> MAPTPKYTFTERAAAGNLSDAEILNSNNPTGSELPDESDVVVGGAGIHGLIYALHASKYKPNNLKISVIEKNTRPGYKIGESTLPIFYTWCKLHGISAAYLLRLFGLKDGLCFYFLDRENQGQYTDFCSVGAPGLVLASLQIERPMSELLFTILAQRNGVNVYHGREVDFKSTVVQGGGQGNKIAVSRGKYDSTPKTIDSALFVDATGRFRQFCSKKAPRHRFDGWNCNAFWGYFTAPKDESKIPFDLYEGDHTNHLCFPEGWVWVIRLPSWEGSPIANLMDMVTYILECADAGVPGDELPSSEELARMFGLKFQWVTSIGFAVRNDVKYPEDLSAYGTREAEQKFNYFVQKYELLQQFMSNFELIENLYGPGTTWFIRKTLAYQSPVVSGPGWLAIGDACGFTNPLYSPGINVGMSTSTWAAQLSHPIVEIGKSAPADAAESSIRKLLVPYDDYCKSLVPALEQMNRFNYVCYRDTRLGPQVACLWQFFAGIDRYLSDVNIETFAHYAIKWVWGAMVPEYQQVAQKCIEHIETVPLDERLPDAMVDELLAFSNRIKSAAVAADDFSLRWDAILRSFDRSLNFVEGKTSRDIYTRQCSGCGAWLQLRPDWKKCHSCGLLGTEPQTAVTFDPP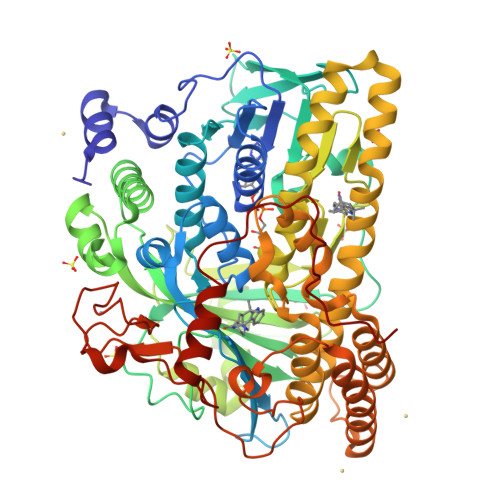LTAEEEALLYAAWNTAPKYDPSKELKLPTPTRPAA>EFSRKTYTLTDYLKNTYRLKLYSLRWISDHEYLYKQENNILVFNAEYGNSSVFLENSTFDEFGHSINDYSISPDGQFILLEYNYVKQWRHSYTASYDIYDLNKRQLITEERIPNNTQWVTWSPVGHKLAYVWNNDIYVKIEPNLPSYRITWTGKEDIIYNGITDWVYEEEVFSAYSALWWSPNGTFLAYAQFNDTEVPLIEYSFYSDESLQYPKTVRVPYPKAGAVNPTVKFFVVNTDSLSSVTNATSIQITAPASMLIGDHYLCDVTWATQERISLQWLRRIQNYSVMDICDYDESSGRWNCLVARQHIEMSTTGWVGRFRPSEPHFTLDGNSFYKIISNEEGYRHICYFQIDKKDCTFITKGTWEVIGIEALTSDYLYYISNEYKGMPGGRNLYKIQLSDYTKVTCLSCELNPERCQYYSVSFSKEAKYYQLRCSGPGLPLYTLHSSVNDKGLRVLEDNSALDKMLQNVQMPSKKLDFIILNETKFWYQMILPPHFDKSKKYPLLLDVYAGPCSQKADTVFRLNWATYLASTENIIVASFDGRGSGYQGDKIMHAINRRLGTFEVEDQIEAARQFSKMGFVDNKRIAIWGWSYGGYVTSMVLGSGSGVFKCGIAVAPVSRWEYYDSVYTERYMGLPTPEDNLDHYRNSTVMSRAENFKQVEYLLIHGTADDNVHFQQSAQISKALVDVGVDFQAMWYTDEDHGIASSTAHQHIYTHMSHFIKQCFSLPHHHHHH[2x]

The dipeptidyl peptidases (DPP) 8 and 9 are serine proteases of the dipeptidyl peptidase 4 activity/structure homologues (DASH) subfamily which cleave post-proline bonds two residues from the N-terminus of a substrate. While DPP4 and FAP are extracellular or secreted proteases, DPP8 and DPP9 are located intracellularly to the cytoplasm and nucleus. There, they play important roles in diverse biological processes such as pyroptosis or ubiquitin-mediated proteolysis, turning them into promising targets for chemical probe and anti-inflammatory or anticancer drug discovery. Here, we show the exploration of the natural product Sulphostin, a DPP4 inhibitor, as a starting point for DPP8/9 inhibitor development.

We therefore also determined an X-ray structure of DPP4 after incubation with Sulphostin, which confirmed the observations made with DPP9. Again, covalent modification of DPP4’s active site serine S630 with a phosphosulfamate group, the product of a nucleophilic attack of the active site serine coupled to a Walden inversion, was exclusively observed, thereby indicating a general covalent reaction mechanism of Sulphostin with DPPs. In agreement with the previous IC50 measurements, these assays confirmed with a kapp of 36,963 M−1 s−1 the preferential binding of Sulphostin to DPP4, followed by DPP9 with a kapp of 317 M−1 s−1 and finally DPP8 with a kapp of 11 M−1 s−1.Destabilase from the medical leech Hirudo medicinalis belongs to the family of i-type lysozymes. It has two different enzymatic activities: microbial cell walls destruction (muramidase activity), and dissolution of the stabilized fibrin (isopeptidase activity). The main difference between low and high salt structures as well as between the two chains of high salt structure is tied to a flexible loop (Gly44-Ser51), containing enzymatically important Asp46. Together with Glu34, Asp46 forms a catalytic dyad for muramidase activity in i-type lysozymes.

To get structural insights into destabilase function we solved its structure in two different crystal forms: P1—obtained at pH 5.0 and high sodium salt concentrations (2.9 M sodium malonate) and P21—obtained at pH 8.0 and low sodium concentration (0.3 M sodium chloride). In the low salt structure, the Gly44-Ser51 loop is bent outward with Asp46 exposed to the bulk solution. Val47 backbone forms a H-bond with an adjacent protein molecule, and therefore crystal packing contributes to stabilization of “open” conformation of the Gly44-Ser51 loop. Our low salt structure lacks the sodium ion but contains cryoprotectant glycerol molecule, H-bonded with Glu34 but not Asp46. Surprisingly, all three amino acid residues in the isopeptidase site of destabilase do not form hydrogen bonds to each other in both high and low salt structures. We expect it is because both our structures were substrate-free.

> QFTDSCLRCICKVEGCDSQIGKCGMDVGSLSCGPYQIKKPYWIDCGKPGGGYESCTKNKACSETCVRAYMKRYGTFCTGGRTPTCQDYARIHNGGPRGCKSSATVGYWNKVQKCLRGTHHHHHH> MKKEPIKMPNPDNTEAYVAGEVAIENSAIALSGIVSVANNADNRLEVFGVSTDSAVWHNWQTAPLPNSSWAGWNKFNGVVTSKPAVHRNSDGRLEVFVRSTDNALWHNWQTAADTNTWSSWQPLYGGITSNPEVC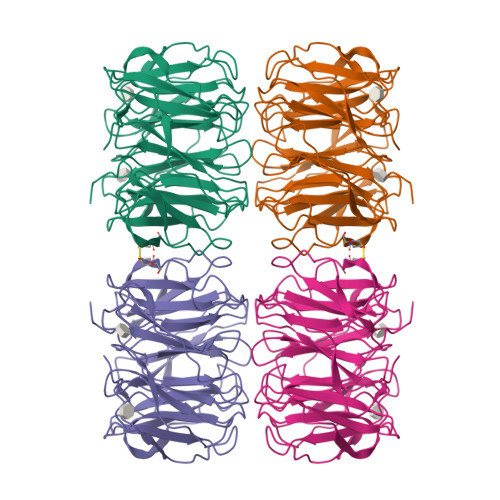LNSDGRLEVFARGTDNALWHIWQTAAHTNSWSNWKSLGGTLTSNPAAHINADGRIEVFARGADNALWHIWQTAAHTDQWSNWQSLKSVITSDPVVIGNCDGRLEVFARGADNTLRHISQIGSDSVSWSNWQCLDGVITSAPAAVKNISGRLEVFARGADNTLWRTWQTSQNGPWSNWSSFTGIIASAPTVAKNSDGRIEVFVLGLDKALWHLWQTTSSTTSSWTTWALIGGITLIDASVIK>MAHHHHHHMPGSELISGGWFREENDQWPGQAMSLRVEKVLYDAPTKFQHLTIFESDPKGPWGTVMALDGCIQVTDYDEFVYHEVLGHTSLCSHPKPERVLIIGGGDGGVLREVLRHGTVEHCDLVDIDGEVMEQSKQHFPQIS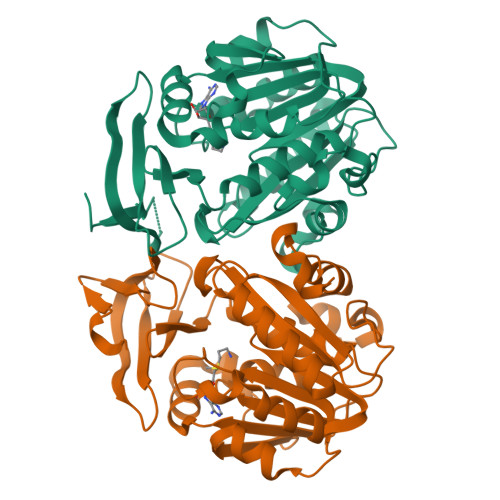RSLADPRATVRVGDGLAFVRQTPDNTYDVVIIDTTDPAGPASKLFGEAFYKDVLRILKPDGICCNQGESIWLDLELIEKMSRFIRETGFASVQYALMHVPTYPCGSIGTLVCSKKAGVDVTKPLRPVEDMPFAKDLKYYDSEMHKASFALPRFARHINNSE[2x]>[2x]G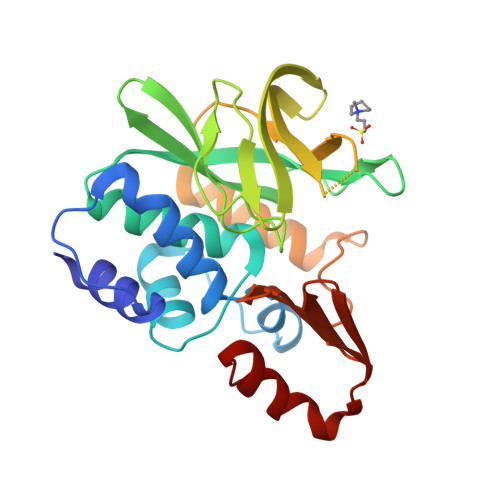SMTDFQKQFFARLHIEEKDTVSFEDLSNIMYAMAQTVPFENLNILEKNFKEISKENLKEKILVNNRGGLCYELNPTMYYFLKDSGFDVHLVSGTVYNAANSIWAVDSGHIATVLTHHNELYLIEVGFGSYLPLAPVPFLGEVIHSATGDYRIRKEMTEKGNYILEMRKNNEFLDQSAADDWTLGYAFYIEEVDEEKANTAQKIIVEHEGSPFNKVPLIVKLTEDGHASLTKDSLTVAKNGKKTKETVTDMQYTNLLHSKFGITL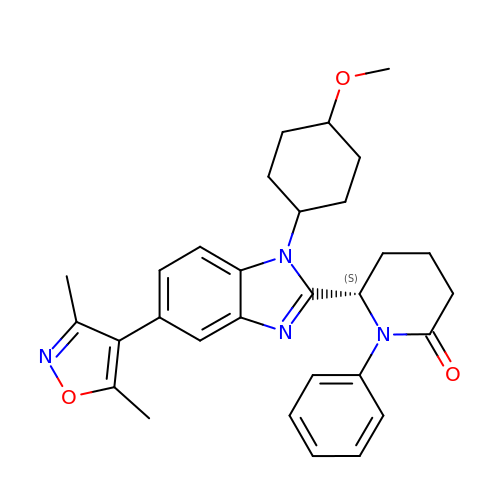(6S)-6-{(5M)-5-(3,5-dimethyl-1,2-oxazol-4-yl)-1-[(1s,4R)-4-methoxycyclohexyl]-1H-benzimidazol-2-yl}-1-phenylpiperidin-2-one | C30 H34 N4 O3 | YQBUUWAEHZBNID-XFAFFCHDSA-N>[2x]GGGG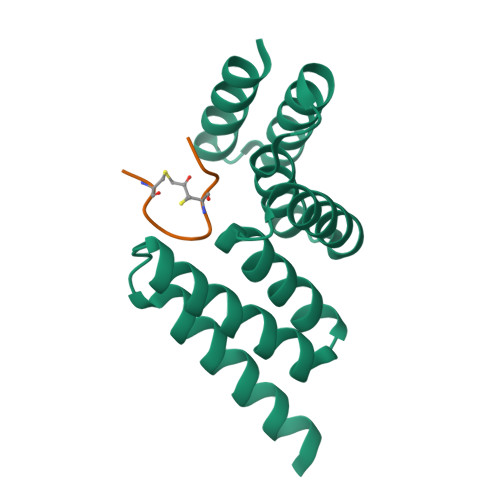GSPEKSPSAQELKEQGNRLFVGRKYPEAAACYGRAITRNPLVAVYYTNRALCYLKMQQHEQALADCRRALELDGQSVKAHFFLGQCQLEMESYDEAIANLQRAYSLAKEQRLNFGDDIPSALRIAKKKRWNSIEER;>ACSSIWCPDG[2x]>[2x]METKPKTATTIKVPPGPLGYVYARACPSEGIELLALLSARSGDSDVAVAPLVVGLTVESGFEANVAVVVGSRTTGLGGTAVSLKLTPSHYSSSVYVFHGGRHLDPSTQAPNLTRLCERARRHFGFSDYTPRPGDLKHETTGEALCERLGLDPDRALLYLVVTEGFKEAVCINNTFLHLGGSDKVTIGGAEVHRIPVYPLQLFMPDFSRVIAEPFNANHRSIGEKFTYPLPFFNRPLNRLLFEAVVGPAAVALRSRNVDAVARAAAHLAFDENHEGAALPADITFTAFEASQGKTPRGGRDGGGKGAAGGFEQRLASVMAGDAALALESIVSMAVFDEPPTDISAWPLFEGQDTAAARANAVGA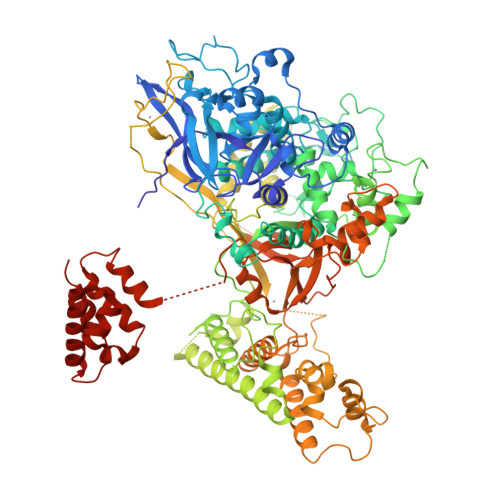YLARAAGLVGAMVFSTNSALHLTEVDDAGPADPKDHSKPSFYRFFLVPGTHVAANPQVDREGHVVPGFEGRPTAPLVGGTQEFAGEHLAMLSGFSPALLAKMLFYLERCDGAVIVGRQEMDVFRYVADSNQTDVPCNLCTFDTRHACVHTTLMRLRARHPKFASAARGAIGVFGTMNSMYSDCDVLGNYAAFSALKRADGSETARTIMQETYRAATERVMAELETLQYVDQAVPTAMGRLETIITNREALHTVVNNVRQVVDREVEQLMRNLVEGRNFKFRDGLGEANHAMSLTLDPYACGPCPLLQLLGRRSNLAVYQDLALSQCHGVFAGQSVEGRNFRNQFQPVLRRRVMDMFNNGFLSAKTLTVALSEGAAICAPSLTAGQTAPAESSFEGDVARVTLGFPKELRVKSRVLFAGASANASEAAKARVASLQSAYQKPDKRVDILLGPLGFLLKQFHAAIFPNGKPPGSNQPNPQWFWTALQRNQLPARLLSREDIETIAFIKKFSLDYGAINFINLAPNNVSELAMYYMANQILRYCDHSTYFINTLTAIIAGSRRPPSVQAAAAWSAQGGAGLEAGARALMDAVDAHPGAWTSMFASCNLLRPVMAARPMVVLGLSISKYYGMAGNDRVFQAGNWASLMGGKNACPLLIFDRTRKFVLACPRAGFVCAASSLGGGAHESSLCEQLRGIISEGGAAVASSVFVATVKSLGPRTQQLQIEDWLALLEDEYLSEEMMELTARALERGNGEWSTDAALEVAHEAEALVSQLG> AECSVDIQGNDQMQFNTNAITVDKSCKQFTVNLSHPGNLPKNVMGHNFVLSTAADMQGVVTDGMASGLDKDFLKPDDSRVIAQTKLIGSGEKDSVTFDVSKLKEGEQFMFFCTFP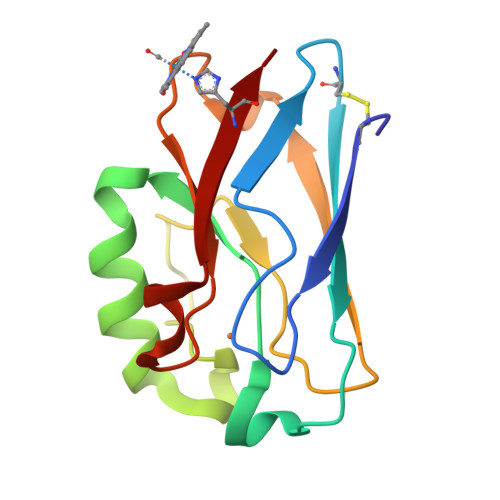GHSALMWGTLHLK> MAEFYGLPN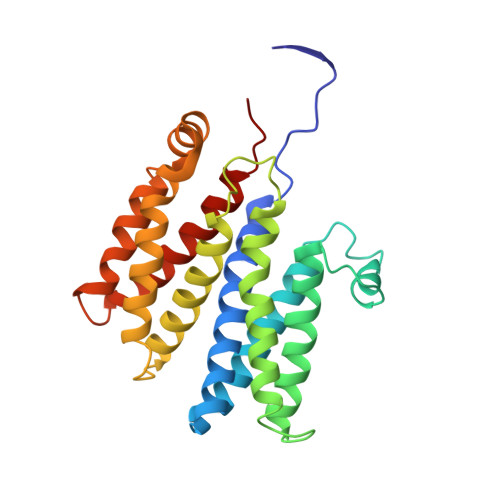AQEFWHWTNALHFVLVGLAGGVALLAALLHLKGDAEARRYTLYALMLIALDLFILWAESPARFRFTHIWLFLSFHPTSPIWWGAWGLGLGFLTGGLLYLGKGSQRALAWALLVFSLVALSYPGLALAVNLNRPLWNGLMAGLFPLTALVLALGLAALLKSPWALFPLRVLAGASLLLALLYPLTLPPEARGHLLEEAGFWYGLFLLLGLGTFWQERLAPWAGLLAAAGLRALLVLAGQWQGLGL>[2x]GPLGSDLIQDVIRRAQENKQRIVLPEGLEPRTLEAADRLMADKVVNIILIGNVDSVKAKVAELGLKNLDEAVIIDPNNHPKKQQYTDLLLQIRQKKGLTPEKAAELVENPLYLGCLIVKSGDADGLIAGAQNTTGDVLRPALQVIKTAPGMTSVSGTFLLFTKAKEYGKDGLLLVADCAVIPNPTADELAQIAVATARTAKAIADIEPRVAMLSFSTKGSAKHEMTDKVVEATRMAQEMAPDLLIDGEMQADAALVERVAALKAPGSNVAGKANVLVFPTLEVGNIAYKLVERLGHAEAVGPILQGMAAPVNDLSRGCSVEDIYRMVAITANQAIAAKEQ

Porphyromonas gingivalis, a black-pigmented Gram-negative rod-type bacterium, is a keystone pathogen linked to the onset and progression of periodontitis. In many bacteria, the enzymes phosphotransacetylase (Pta, EC 2.3.1.8) and acetate kinase (Ack, EC 2.7.2.1) form a key pathway for production of ATP from excess acetyl coenzyme A (acetyl-CoA). Pta produces acetyl phosphate (AcP) from acetyl-CoA, and AcP is subsequently converted to acetate by Ack, with the concomitant production of ATP through substrate-level phosphorylation. In the current study, recombinant Pta (PgPta) and Ack (PgAck) from P. gingivalis ATCC 33277, encoded by pta (PGN_1179) and ack (PGN_1178), respectively, were prepared and enzymatically characterized.

Structural and mutational analyses suggest that Pta is a dimer with two substrate-binding sites in each subunit. Six amino acid residues (Arg89, Arg135, Asp309, Ser311, Arg312, and Asp318) positioned at the cleft and the acetyl-CoA binding site were mutated and recombinant proteins were prepared to investigate their contributions to catalytic activity. The polypeptide region in which Asp309, Ser311, and Arg312 are located forms part of the side of the cleft on the domain I side, with Ser311 and Arg312 positioned at the edge of the cleft, and Asp309 located near the bottom of the cleft. Mutation of these residues resulted in the complete loss of enzyme activity. Finally, Asp318 is located at the edge of the cleft on the opposite side from the observed acetyl-CoA binding site. The D318A mutant displayed only 11% of the specific activity of the WT enzyme.> AQQMPSLAPMLEKVMPSVVSINVEGSTTVNTPRM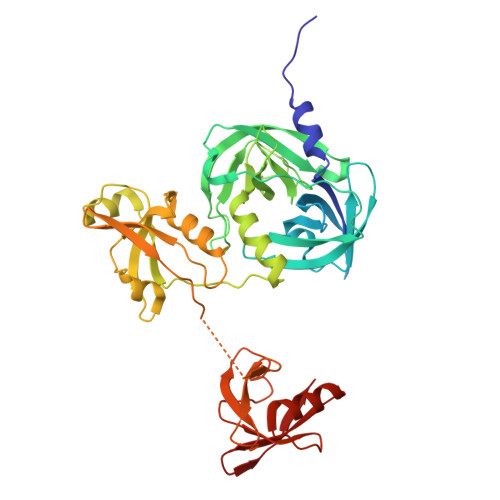PRNFQQFFGDDSPFCQEGSPFQSSPFCQGGQGGNGGGQQQKFMALGSGVIIDADKGYVVTNNHVVDNATVIKVQLSDGRKFDAKMVGKDPRSDIALIQIQNPKNLTAIKMADSDALRVGDYTVAIGNPFGLGETVTSGIVSALGRSGLNAENYENFIQTDAAINRGNAGGALVNLNGELIGINTAILAPDGGNIGIGFAIPSNMVKNLTSQMVEYGQVKRGELGIMGTELNSELAKAMKVDAQRGAFVSQVLPNSSAAKAGIKAGDVITSLNGKPISSFAALRAQVGTMPVGSKLTLGLLRDGKQVNVNLELQQSSQNQVDSSSIFNGIEGAEMSNKGKDQGVVVNNVKTGTPAAQIGLKKGDVIIGANQQAVKNIAELRKVLDSKPSVLALNIQRGDSTIYLLMQ> MMTTPELSCDVLIIGSGAAGLSLALRLAEKHKVIVLSKGPVSEGSTFYAQGGIAAVFDETDSIASHVEDTLIAGAGICDRHAVEFVASNARTCVQWLIDQGVLFDTHVQPNGKESYHLTREGGHSHRRILHAADATGKEVETTLVSRAQNHPNIQVLE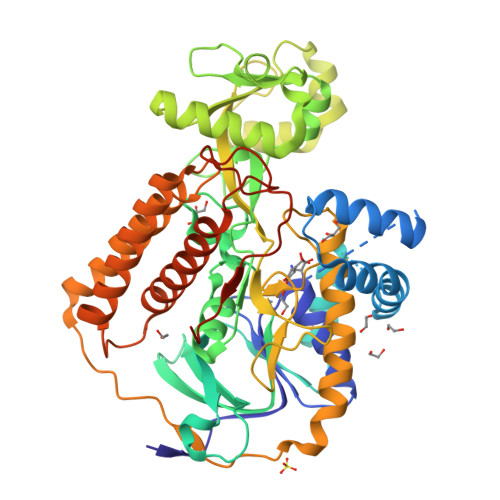RSNAVDLIISDKMGLPGPRRVVGAWIWNRNKEWVETCHAKSVVLATGGASKVYQYTTNPDISSGDGIAMAWRAGCRVANLEFNQFHPTALYHPQARNFLLTEALRGEGAYLKRPDGSRFMPDVDERGELAPRDIVARAIDHEMKQLGADCMFLDISHKPDDFVRQHFPMIYAKLLDLGMDLTKEPIPVVPAAHYTCGGVVVDDYGRTDVDGLYAIGEVSYTGLHGANRMASNSLLECLVYGWSAAMDIDRRMPSVHSVDALPAWDESRVENADERVVIQHNWHELRLLMWDYVGIVRTTKRLERALRRITMLQQEIDEYYANFRVSNNLLELRNLVQVAELIVRCAMMRKESRGLHFTLDYPQQLAESGPSILSPLTPHINRRGENLYFQSAGHHHHHH~{N}-(4-azanylbutyl)-~{N}-(2-azanyl-2-oxidanylidene-ethyl)-7-(3-azanyl-3-oxidanylidene-propyl)-4-(dimethylamino)-2-(2-naphthalen-2-ylethylamino)pyrrolo[2,3-d]pyrimidine-6-carboxamide 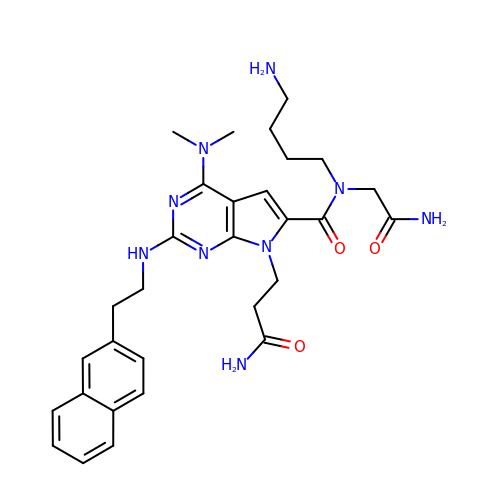| C30 H39 N9 O3 | WDNXQKSPKHPWGU-UHFFFAOYSA-N>[25x]GDNQDRTVANTQPSGPSNSTEIPALTAVETGHTSQVDPSDTIQTRHVVNFHSRSESTIENFMGRAACVFMDQYKINGEETSTDRFAVWTINIREMAQLRRKCEMFTYMRFDIEMTMVITSCQDQGTILDQDMPVLTHQIMYVPPGGPIPAKVDGYEWQTSTNPSVFWTEGNAPPRISIPFISVGNAYSSFYDGWSHFTQDGTYGYTTLNAMGKLYIRHVNRSSPHQITSTIRVYFKPKHIKAWVPRPPRLCPYINKRDVNFVVTEITDSRTSITDTPHPEHSVLATH;>[25x]SPSAEECGYSDRVRSMTLGNSTITTQESANVVVGYGEWPSYLSDREATAEDQPTQPDVATCRFYTLESVQWEKTSPGWWWKFPEALKNMGLFGQNMHYHYLGRAGYTIHVQCNASKFHQGCLLVVCVPEAEMGCADTDTTFPATELTTEDTPHVFTSDSIT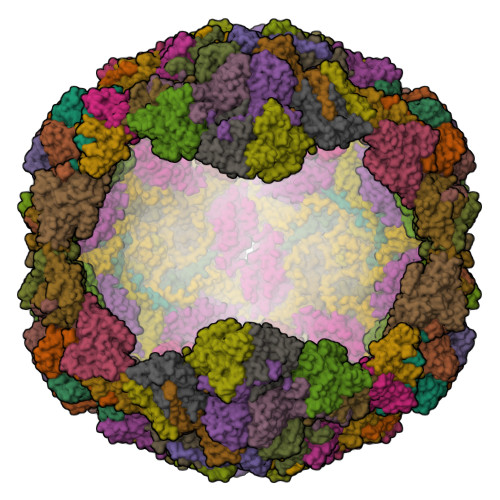GKKVQAAVCNAGMGVGVGNLTIFPHQWINLRTNNSATIVIPYINSVPMDNMFRHYNFTLMIIPFAPLNFTDGATAYVPITVTIAPMYAEYNGLRLASTQ;>[25x]GVPVLNTPGSNQFLTSDDYQSPSAMPQFDETPEMHIPGEVRNLMEIAEVDSVVPVNNVTGKTKSMDAYQIPVGTGNTDKTKPIFSFQMDPGYSSVLKRTLLGEMLNYYAHWSGSVKLTFLFCGSAMATGKLLISYSPPGASVPTSRKDAMLGTHIVWDIGLQSSCVLCVPWISQSHYRMVQQDPYTSAGYITCWYQTNIVVPPGAPTSCDVLCFASACNDFSVRLLRDTPFMAQPGKLQ> MNSDYILQHADALVKRVSKLIVNEPAARAALRRGVGLAPEDPRMLAAHRVVAPYVPVPTDYDVDRRRAASLWDVHAVERAFYAVAAIMAAQPRSARDQEAEATEEQTGEPQDSEALTEPTPAEESSATKDGK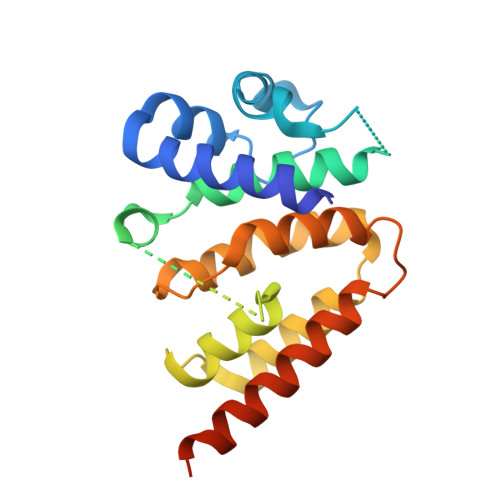PDRRPNLGVSLAQAVFDKGLNADSTEQRLHLIARQNLDGVHRHLPRLVLYLRSDQVHIDWGILIRDLARWGHTPRHVAREWVQDYHRTLETLTRQAEQKNKNNTTDEEAEAA> HHHHHHNAVEIQGVSQRYGSMTVLHDLNLNLGEGEVLGLFGHNGAGKTTSMKLILGLL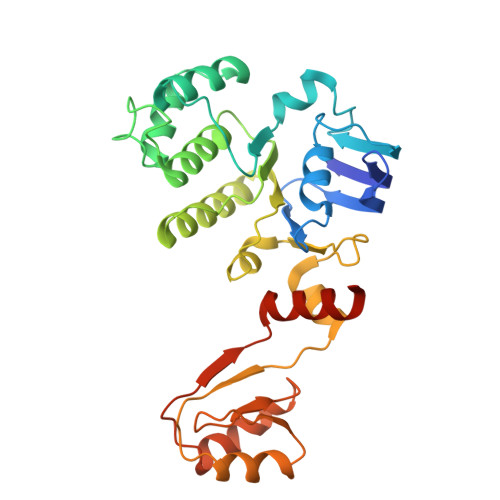SPSEGQVKVLGRAPNDPQVRRQLGYLPENVTFYPQLSGRETLRHFARLKGAALTQVDELLEQVGLAHAADRRVKTYSKGMRQRLGLAQALLGEPRLLLLDQPTVGLDPIATQDLYLLIDRLRQRGTSIILCSHVLPGVEAHINRAAILAKGCLQAVGSLSQLRAEAGLPVRIRASGISERDSWLQRWTDAGHSARGLSESSIEVVAVNGHKLVLLRQLLGEGEPEDIEIHQPSLEDLYRYYMERAGDVRAQEGRL>[2x]SHRYVETMLVADQSMAEFHGSGLKHYLLTLFSVAARLYKHPSIRNSVSLVVVKILVIHDEQKGPEVTSNAALTLRNFCNWQKQHNPPSDRDAE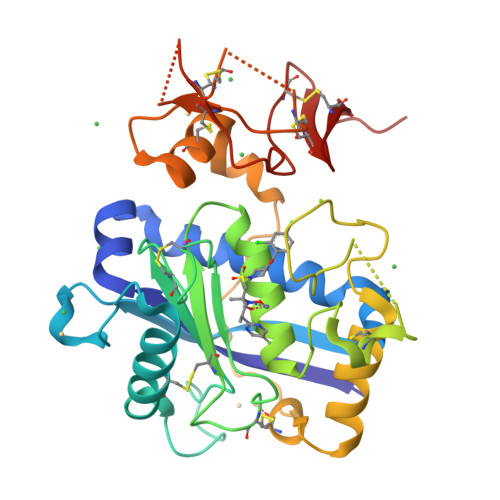HYDTAILFTRQDLCGSQTCDTLGMADVGTVCDPSRSCSVIEDDGLQAAFTTAHELGHVFNMPHDDAKQCASLNGVNQDSHMMASMLSNLDHSQPWSPCSAYMITSFLDNGHGECLMDKPQNPIQLPGDLPGTSYDANRQCQFTFGEDSKHCPDAASTCSTLWCTGTSGGVLVCQTKHFPWADGTSCGEGKWCINGKCVNKLVPR>MDKLAVLYAEHIATLQQRTRTITEREGLEGLVIHSGQAKRQFLDWMYYPFKVNPQFKAWLPVIDNPHCWIVVDGASKPKLIFYRPVDFWHKVPDEPRDFWAEYFDIELLVQPDQVEKLLPYDKANYAYIGEYLEVAQALGFSIMNPEPVMNYLHFHRAYKTQYELECLRQANRIAVEGHKAARDTFFNGGSEFDIQHAYLMATRQSENEMPYGNIVALNENCAILGYTHFEPTAPHTHHSFLIDAGANFNGYAADITRTYDFKKSGEFSDLIQVMTEHQIALGKALKPGLLYGELHLECHQRVAQVLSDFNIVKLPAADIVERGITSTF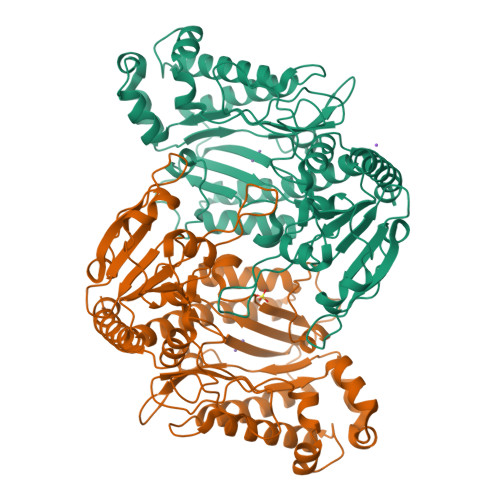FPHGLGHHLGLQVHDMGGFMADESGTHQAPPEGHPFLRCTRLIEKNQVFTIEPGLYFIDSLLGDLAQTDNKQFINWEKVEEFKPFGGIRIEDNIIVHEDSLENMTRDLHLDLDHHHHHH[4x]> GVPTYLLPGS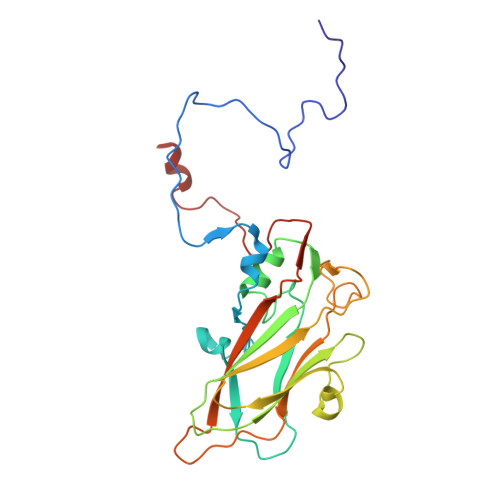GQFLTTDDHSSAPVLPCFNPTPEMHIPGQIRNMLEMIQVESMMEINNTDGANGMERLRVDISVQADLDQLLFNIPLDIQLDGPLRNTLVGNISRYYTHWSGSLEMTFMFCGSFMATGKLILCYTPPGGSCPTTRETAMLGTHIVWDFGLQSSITLIIPWISGSHYRMFNSDAKSTNANVGYVTCFMQTNLIVPSESSDTCSLIGFIAAKDDFSLRLMRDSPDIGQSNHLHGAEAAYQ> GAACGACACTGA;> CGGCGACTC;> TCACCG;> TCGAGTCGGTGT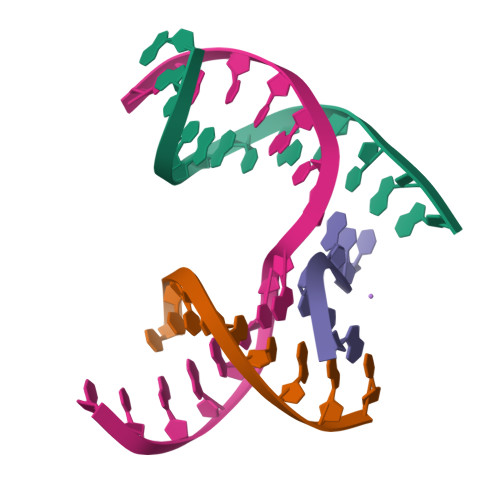CGT Mtb FAS-I is an α6 subtype complex, composed of six long polypeptide chains with an overall molecular weight of ~2 MDa. Each of the α chains has seven catalytic domains and is 3069 amino acids long. The mycobacterial FAS-I has a distinct capacity to elongate fatty acids beyond C16, to C24/267,8, which are further elongated to meromycolate (C56) by the FAS-II system and then condensed with C26 to form mycolic acids. Here we report the 3.3 Å resolution structure of the ~2 MDa FAS-I from Mtb, determined by single particle cryo-EM.

A 3D map with D3 symmetry imposed was reconstructed from a final data set of 40,160 particles at 3.3 Å overall resolution with good angular coverage. Out of seven functional domains of Mtb FAS-I, we modeled the six domains that make the barrel-like cage. The density for the ACP was weak and thus we did not model it (see Methods section). The localized reconstruction revealed orientations of the ACP which were not observed in the context of the whole complex, however the resolution of the ACP within the sub-particle classes was similar to that obtained using 3D classification of the whole complex. This indicates that the ACP domains are not rigidly held in a single position within the chamber but rather occupy a continuum of closely related orientations and possibly conformations. Putative docking of ACP domains to the KS modules is partially mediated by a long loop (residues 2210–2226) that projects from the neighboring ketoacyl reductase (KR) module (KR-loop). Negatively charged surfaces are also found near the catalytic sites of the acetyltransferase (AT), ER, dehydratase (DH), and KR modules, suggesting that in the case of Mtb FAS-I electrostatic interactions may also mediate attachment of ACP to the catalytic modules but with an opposite charge as in the fungal FAS-I system. The catalytic cleft of the ER from Mtb FAS-I is wider compared to the fungal-ER, and the flavin mononucleotide (FMN) co-factor in Mtb FAS-I is more exposed compared to the FMN in the fungal FAS-I. This difference is mostly due to the local amino acid composition rather than changes in backbone conformation. The catalytic cleft of the KR module is also much wider in Mtb FAS-I compared to fungal FAS-I. More striking is the larger inner volume of the Mtb DH catalytic chamber compared to the fungal protein. The extended catalytic clefts of the KR, DH, and ER modules may reflect evolutionary adaptation of Mtb FAS-I for producing the unusually long C26 fatty acids; larger clefts are probably required for accommodating the longer aliphatic chains, while the ACP-attached pantothenic acid reaches into the active sites.

>MKKWSHPQFEKGGSDYKDDDDKPICTIHEHDRVSADRGGDSPHTTHALVDRLMAGEPYAVAFGGQGSAWLETLEELVSATGIETELATLVGEAELLLDPVTDELIVVRPIGFEPLQWVRALAAEDPVPSDKHLTSAAVSVPGVLLTQIAATRALARQGMDLVATPPVAMAGHSQGVLAVEALKAGGARDVELFALAQLIGAAGTLVARRRGISVLGDRPPMVSVTNADPERIGRLLDEFAQDVRTVLPPVLSIRNGRRAVVITGTPEQLSRFELYCRQISEKEEADRKNKVRGGDVFSPVFEPVQVEVGFHTPRLSDGIDIVAGWAEKAGLDVALARELADAILIRKVDWVDEITRVHAAGARWILDLGPGDILTRLTAPVIRGLGIGIVPAATRGGQRNLFTVGATPEVARAWSSYAPTVVRLPDGRVKLSTKFTRLTGRSPILLAGMTPTTVDAKIVAAAANAGHWAELAGGGQVTEEIFGNRIEQMAGLLEPGRTYQFNALFLDPYLWKLQVGGKRLVQKARQSGAAIDGVVISAGIPDLDEAVELIDELGDIGISHVVFKPGTIEQIRSVIRIATEVPTKPVIMHVEGGRAGGHHSWEDLDDLLLATYSELRSRANITVCVGGGIGTPRRAAEYLSGRWAQAYGFPLMPIDGILVGTAAMATKESTTSPSVKRMLVDTQGTDQWISAGKAQGGMASSRSQLGADIHEIDNSASRCGRLLDEVAGDAEAVAERRDEIIAAMAKTAKPYFGDVADMTYLQWLRRYVELAIGEGNSTADTASVGSPWLADTWRDRFEQMLQRAEARLHPQDFGPIQTLFTDAGLLDNPQQAIAALLARYPDAETVQLHPADVPFFVTLCKTLGKPVNFVPVIDQDVRRWWRSDSLWQAHDARYDADAVCIIPGTASVAGITRMDEPVGELLDRFEQAAIDEVLGAGVEPKDVASRRLGRADVAGPLAVVLDAPDVRWAGRTVTNPVHRIADPAEWQVHDGPENPRATHSSTGARLQTHGDDVALSVPVSGTWVDIRFTLPANTVDGGTPVIATEDATSAMRTVLAIAAGVDSPEFLPAVANGTATLTVDWHPERVADHTGVTATFGEPLAPSLTNVPDALVGPCWPAVFAAIGSAVTDTGEPVVEGLLSLVHLDHAARVVGQLPTVPAQLTVTATAANATDTDMGRVVPVSVVVTGADGAVIATLEERFAILGRTGSAELADPARAGGAVSANATDTPRRRRRDVTITAPVDMRPFAVVSGDHNPIHTDRAAALLAGLESPIVHGMWLSAAAQHAVTATDGQARPPARLVGWTARFLGMVRPGDEVDFRVERVGIDQGAEIVDVAARVGSDLVMSASARLAAPKTVYAFPGQGIQHKGMGMEVRARSKAARKVWDTADKFTRDTLGFSVLHVVRDNPTSIIASGVHYHHPDGVLYLTQFTQVAMATVAAAQVAEMREQGAFVEGAIACGHSVGEYTALACVTGIYQLEALLEMVFHRGSKMHDIVPRDELGRSNYRLAAIRPSQIDLDDADVPAFVAGIAESTGEFLEIVNFNLRGSQYAIAGTVRGLEALEAEVERRRELTGGRRSFILVPGIDVPFHSRVLRVGVAEFRRSLDRVMPRDADPDLIIGRYIPNLVPRLFTLDRDFIQEIRDLVPAEPLDEILADYDTWLRERPREMARTVFIELLAWQFASPVRWIETQDLLFIEEAAGGLGVERFVEIGVKSSPTVAGLATNTLKLPEYAHSTVEVLNAERDAAVLFATDTDPEPEPEEDEPVAESPAPDVVSEAAPVAPAASSAGPRPDDLVFDAADATLALIALSAKMRIDQIEELDSIESITDGASSRRNQLLVDLGSELNLGAIDGAAESDLAGLRSQVTKLARTYKPYGPVLSDAINDQLRTVLGPSGKRPGAIAERVKKTWELGEGWAKHVTVEVALGTREGSSVRGGAMGHLHEGALADAASVDKVIDAAVASVAARQGVSVALPSAGSGGGATIDAAALSEFTDQITGREGVLASAARLVLGQLGLDDPVNALPAAPDSELIDLVTAELGADWPRLVAPVFDPKKAVVFDDRWASAREDLVKLWLTDEGDIDADWPRLAERFEGAGHVVATQATWWQGKSLAAGRQIHASLYGRIAAGAENPEPGRYGGEVAVVTGASKGSIAASVVARLLDGGATVIATTSKLDEERLAFYRTLYRDHARYGAALWLVAANMASYSDVDALVEWIGTEQTESLGPQSIHIKDAQTPTLLFPFAAPRVVGDLSEAGSRAEMEMKVLLWAVQRLIGGLSTIGAERDIASRLHVVLPGSPNRGMFGGDGAYGEAKSALDAVVSRWHAESSWAARVSLAHALIGWTRGTGLMGHNDAIVAAVEEAGVTTYSTDEMAALLLDLCDAESKVAAARSPIKADLTGGLAEANLDMAELAAKAREQMSAAAAVDEDAEAPGAIAALPSPPRGFTPAPPPQWDDLDVDPADLVVIVGGAEIGPYGSSRTRFEMEVENELSAAGVLELAWTTGLIRWEDDPQPGWYDTESGEMVDESELVQRYHDAVVQRVGIREFVDDGAIDPDHASPLLVSVFLEKDFAFVVSSEADARAFVEFDPEHTVIRPVPDSTDWQVIRKAGTEIRVPRKTKLSRVVGGQIPTGFDPTVWGISADMAGSIDRLAVWNMVATVDAFLSSGFSPAEVMRYVHPSLVANTQGTGMGGGTSMQTMYHGNLLGRNKPNDIFQEVLPNIIAAHVVQSYVGSYGAMIHPVAACATAAVSVEEGVDKIRLGKAQLVVAGGLDDLTLEGIIGFGDMAATADTSMMCGRGIHDSKFSRPNDRRRLGFVEAQGGGTILLARGDLALRMGLPVLAVVAFAQSFGDGVHTSIPAPGLGALGAGRGGKDSPLARALAKLGVAADDVAVISKHDTSTLANDPNETELHERLADALGRSEGAPLFVVSQKSLTGHAKGGAAVFQMMGLCQILRDGVIPPNRSLDCVDDELAGSAHFVWVRDTLRLGGKFPLKAGMLTSLGFGHVSGLVALVHPQAFIASLDPAQRADYQRRADARLLAGQRRLASAIAGGAPMYQRPGDRRFDHHAPERPQEASMLLNPAARLGDGEAYI[6x]[(2R,3S,4R,5R)-5-(2-amino-6-oxo-1,6-dihydro-9H-purin-9-yl)-3,4-dihydroxyoxolan-2-yl]methyl (2R,3S,4R,5R,6S)-6-[(1R)-1,2-dihydroxyethyl]-3,4,5-trihydroxyoxan-2-yl dihydrogen diphosphate (non-preferred name) | C17 H27 N5 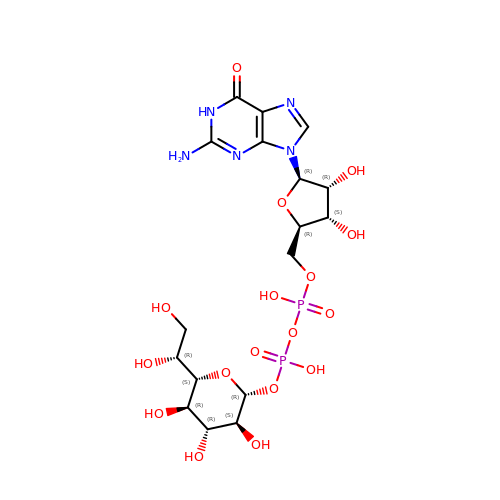O17 P2 | HRUXIQZFNLQZQA-GVGRRHNDSA-N> GSETQQVPTEEVSLEVLLSNGQKVLVNVLTSDQTEDVLEAVAAKLDLPDDLIGYFSLFLVREKEDGAFS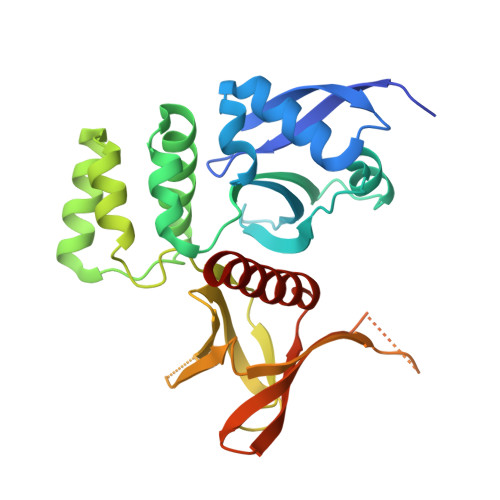FVRKLQEFELPYVSVTSLRSQEYKIVLRKSYWDSAYDDDVMENRVGLNLLYAQTVSDIERGWILVTKEQHRQLKSLQEKVSKKEFLRLAQTLRHYGYLRFDACVADFPEKDCPVVVSAGNSELSLQLRLPGQQLREGSFRVTRMRCWRVTSSVPLPSGSTSSPGRGRGEVRLELAFEYLMSKDRLQWVTITSPQAIMMSICLQSMVDELMVKKSGGS>[4x]MHHHHHHVKLQLVAVGTKMPDWVQTGFTEYLRRFPKDMPFELIEIPAGKRGKNADIKRILD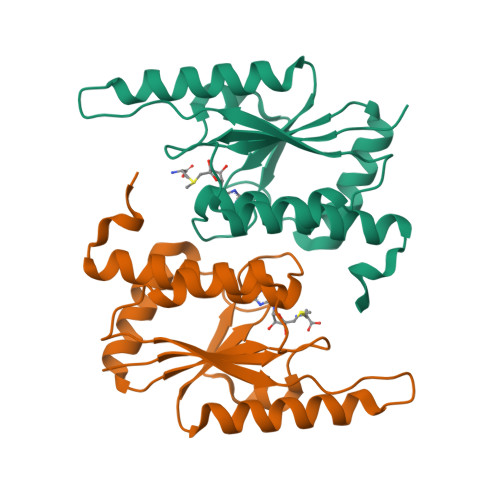KEGEQMLAAAGKNRIVTLDIPGKPWDTPQLAAELERWKLDGRDVSLLIGGPEGLSPACKAAAEQSWSLSALTLPHPLVRVLVAESLYRAWSITTNHPYHRE> EPEPWFFKNLSRKDAERQLLAPGNTHGSFLIRESESTAGSFSLSVRDFDQNQGEVVKHYKIRNLDNGGFYISPRITFPGLHELVRHYT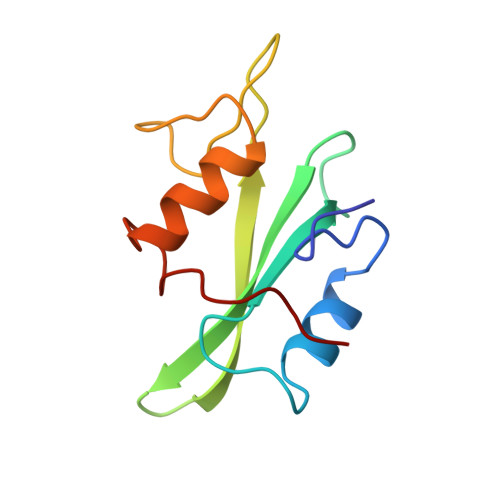NASDGLCTRLSRPCQT> MSATKSIVGEALEYVNIGLSHFLALPLAQRISLIIIIPFIYNIVWQLLYSLRKDRPPLVFYWIPWVGSAVVYGMKPYEFFEECQKKYGDIFSFVLLGRVMTVYLGPKGHEFVFNAKLADVSAEAAYAHLTTPVFGKGVIYDCPNSRLMEQKKFVKGALTKEAFKSYVPLIAEEVYKYFRDSKNFRLNERTTGTIDVMVTQPEMTIFTASRSLLGKEMRAKLDTDFAYLYSDLDKGFTPINFVFPNLPLEHYRKRDHAQKAISGTYMSLIKERRKNNDIQDRDLIDSLMKNSTYKDGVKMTDQEIA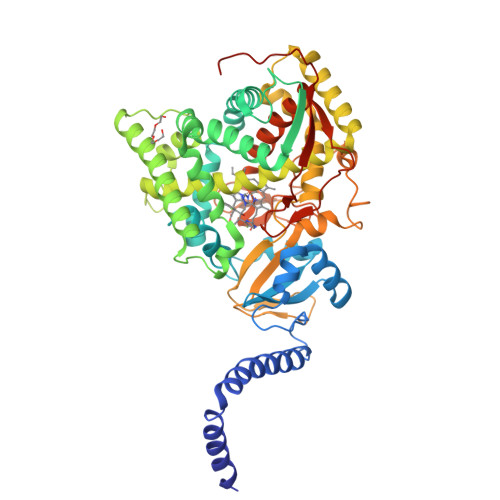NLLIGVLMGGQHTSAATSAWILLHLAERPDVQQELYEEQMRVLDGGKKELTYDLLQEMPLLNQTIKETLRMHHPLHSLFRKVMKDMHVPNTSYVIPAGYHVLVSPGYTHLRDEYFPNAHQFNIHRWNNDSASSYSVGEEVDYGFGAISKGVSSPYLPFGGGRHRCTGEHFAYCQLGVLMSIFIRTLKWHYPEGKTVPPPDFTSMVTLPTGPAKIIWEKRNPEQKIGGRHHHHHH>MLNTQTIIDVNKAMDAMLRAYLNQDIAIRFDLPELDTMQSDAMVSIFLYDIHEDLQLRSAESRGFDVYAGRLLPGWVNIKCNYLITYWEASKPATDASSPDSQPDNQAIQVMSQVLNALINNRQLAGIPGAYTQVVPPKESLNSLGNFWQSLGNRPRLSLNYSVTVPVSLNDGQDSATPVTAVSSTVEQTASLSQEVVSHALRELLITELGGGEDNRLVLSKVELSAVKETMTQDSPAQMIILLSVSGITRQEYLKEIDNIFDRWVNNAEVITTIDDCGIRIESITKDNLVGI[6x];>MSTSTSQIAVEYPIPVYRFIVSVGDEKIPFNSVSGLDISYDTIEYRDGVGNWFKMPGQSQSTNITLRKGVFPGKT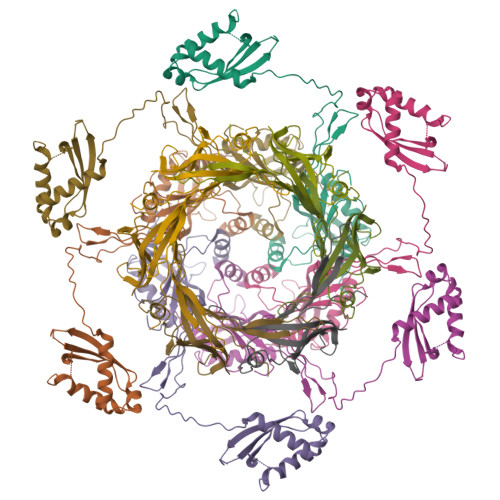ELFDWINSIQLNQVEKKDITISLTNDAGTELLMTWNVSNAFPTSLTSPSFDATSNDIAVQEITLMADRVIMQAV[6x]> STTLTRQDLNFGQVVADVLCEFLEVAVHLILYVREVYPVGIFQKRKKYNVPVQMSCHPELNQY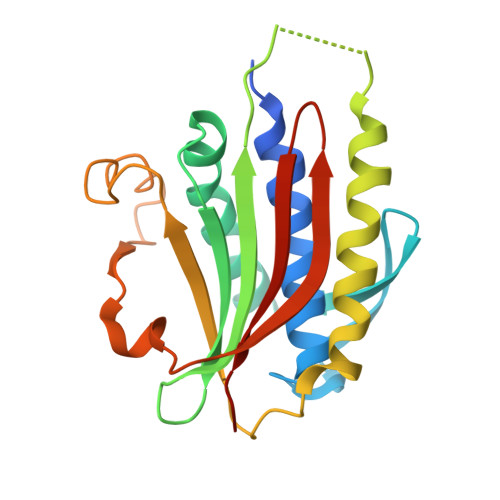IQDTLHCVKPLLEKNDVEKVVVVILDKEHRPVEKFVFEITQPPLLSISSDSLLSHVEQLLRAFILKISVCDAVLDHNPPGCTFTVLVHTREAATRNMEKIQVIKDFPWILADEQDVHMHDPRLIPLKTMTSDILKMQLYVEERAHKGS Carboxylesterases are a family of enzymes that act on a variety of both exogenous (e.g. cocaine, heroin) and endogenous (e.g. acyl-CoA esters) substrates. They are defined by their ability to hydrolyze ester, amide, or thioester bonds to their corresponding alcohol, amine or thiol and free acid in a diverse range of chemically distinct compounds. Carboxylesterases comprise three distinct domains; a central domain containing the catalytic triad (S221, H467 and E354), a regulatory domain (RD) and an α/β domain. The active site occupies a 10-15Å deep hydrophobic pocket at the interface of the three domains with all three catalytic residues arranged such that a proton transfer chain can be established.

The structure-function relationship of this aglycosylated hCES1 was explored alongside the wild type enzyme and a catalytically inactive mutant (S221A). Here, recombinant hCES1 enzymes were produced in HEK293 cells using either transient expression (hCES1 N79Q) or from stable cell lines (hCES1 and S221A). The HEK Gnt1-/- mutant cell line in which N-glycosylation is restricted to GlcNAc2Man5 was used for generating stable cell lines. In all three structures, the asymmetric unit contained one monomer of hCES1, containing, two disulphide bridges were present, C87- C116 and C274—C285 as seen in other hCES1 structures. In the crystal structure of hCES1 and hCES1 S221A, an N-acetylglucosamine adduct was observed attached to the side chain of residue N79. Space group symmetry was used to generate the biological trimer that is seen in solution. Superposition of the monomeric structures showed no differences between the glycosylated and aglycosylated hCES1. The orientation of the side-chains of the catalytic triad (S221, E354, H467) in bound and unbound enzymes was also identical showing that the enzyme is pre-disposed for substrate binding.

> SSPPVVDTVHGKVLGKFVSLEGFAQPVAIFLGIPFAKPPLGPLRFTPPQPAEPWSFVKNATSYPPMCTQDPKAGQLLSELFTNRKENIPLKLSEDCLYLNIYTPADLTKKNRLPVMVWIHGGGLMVGAASTYDGLALAAHENVVVVTIQYRLGIWGFFSTGDEHSRGNWGHLDQVAALRWVQDNIASFGGNPGSVTIFGESAGGESVSVLVLSPLAKNLFHRAISESGVALTSVLVKKGDVKPLAEQIAITAGCKTTTSAVMVHCLRQKTEEELLETTLKMKFLSLDLQGDPRESQPLLGTVIDGMLLLKTPEELQAERNFHTVPYMVGINKQEFGWLIPMLMSYPLSEGQLDQKTAMSLLWKSYPLVCIAKELIPEATEKYLGGTDDTVKKKDLFLDLIADVMFGVPSVIVARNHRDAGAPTYMYEFQYRPSFSSDMKPKTVIGDHGDELFSVFGAPFLKEGASEEEIRLSKMVMKFWANFARNGNPNGEGLPHWPEYNQKEGYLQIGANTQAAQKLKDKEVAFWTNLFAK>GPGSTYIFSKGGGQITYKWPPNDRPSTRADRLAIGFSTVQKEAVLVRVDSSSGLGDYLELHIHQGKIGVKFNVGTDDIAIEESNAIINDGKYHVVRFTRSGGNATLQVDSWPVIERYPAGNNDNERLAIARQRIPYRLGRVVDEWLLDKGRQLTIFNSQATIIIGGKEQGQPFQGQLSGLYYNGLKVLNMAAEN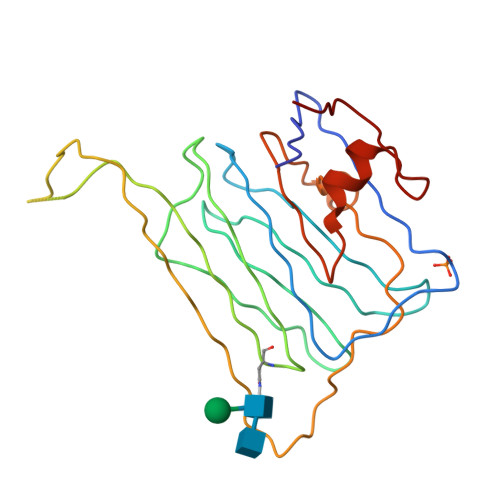DANIAIVGNVRLV[2x]>MFENITAAPADPILGLADLFRADERPGKINLGIGVYKDETGKTPVLTSVKKAEQYLLENETTKNYLGIDGIPEFGRCTQELLFGKGSALINDKRARTAQTPGGTGALRVAADFLAKNTSVKRVWVSNPSWPNHKSVFNSAGLEVREYAYYDAENHTLDFDALINSLNEAQAGDVVLFHGCCHNATGIDPTLEQWQTLAQLSVEKGWLPLFDFAYQGFARGLEEDAEGLRAFAAMHKELIVASSYSKNFGLYNERVGACTLVAADSETVDRAFSQMKAAIRANYSNPPAHGASVVATILSNDALRAIWEQELTDMR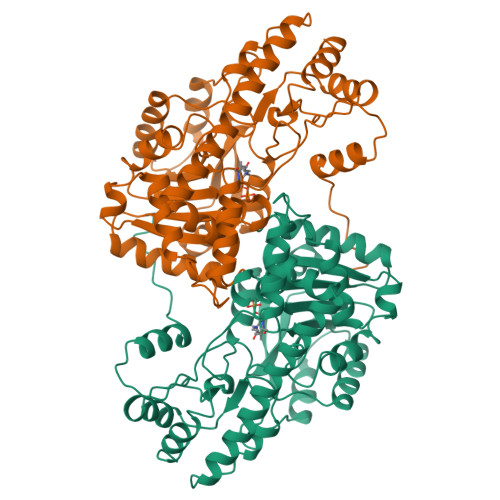QRIQRMRQLFVNTLQEKGANRDFSFIIKQNGMFSFSGLTKEQVLRLREEFGVYAVASGRVNVAGMTPDNMAPLCEAIVAVL[2x]> GSKMEE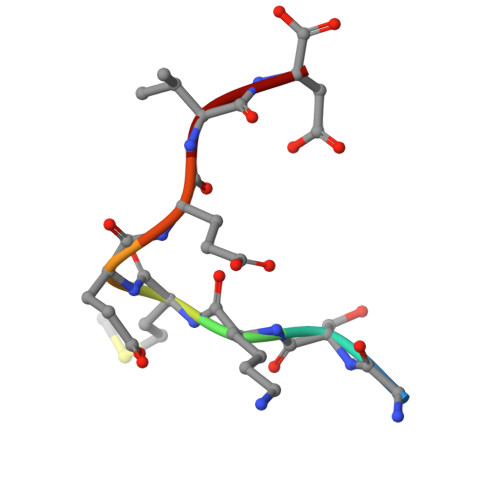VD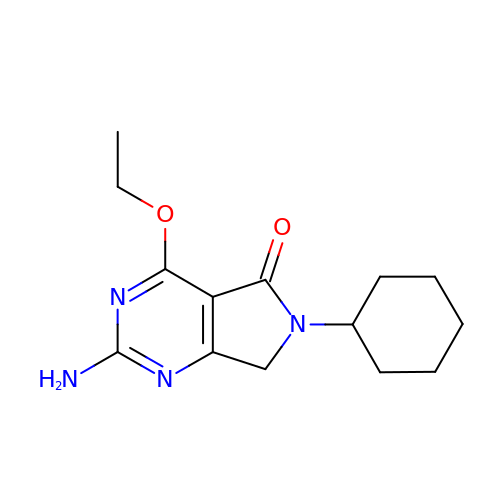2-azanyl-6-cyclohexyl-4-ethoxy-7~{H}-pyrrolo[3,4-d]pyrimidin-5-one | C14 H20 N4 O2 | OHMOSKPEUXXALI-UHFFFAOYSA-N> MAPALVQRRKKVAMIGSGMI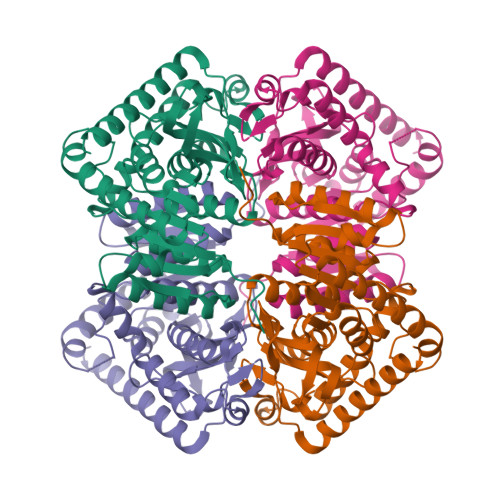GGTMGYLCALRELADVVLYDVVKGMPEGKALDLSHVTSVVDTNVSVRAEYSYEAALTGADCVIVTAGLTKVPGKPDSEWSRNDLLPFNSKIIREIGQNIKKYCPKTFIIVVTNPLDCMVKVMCEASGVPTNMICGMACMLDSGRFRRYVADALSVSPRDVQATVIGTHGDCMVPLVRYITVNGYPIQKFIKDGVVTEKQLEEIAEHTKVSGGEIVRFLGQGSAYYAPAASAVAMATSFLNDEKRVIPCSVYCNGEYGLKDMFIGLPAVIGGAGIERVIELELNEEEKKQFQKSVDDVMALNKAVAALQAPG> EHRVLHLRDRLDLAAELKLLCERGPLVRIPLEDGSAVHWFALGYDVVREVLGSEKFDKRVIGTHFNHQEMALPGNLLQLDPPEHTRLRRMVAPAYSVRRMQALEPRVQAIVDDHLDTMASTGPPVEFLREVAGPMAARVACEFLGIPLDDRGELIRLTAHRGGKRRRVLNGHAYLAYMRELAARLRRDPGDGMLGMVARDHGADISDEELAGLCAVVMNSSVEQTESCLAAGTLLLLEHPEQFALLRERPELGEQAVEEIVRYLSVFEGLDPRTATEDVEIGGQVIKKGEAVFCSLLAANRADPALDGFDITRKESRHVAFGHGIHHCLGAPLARMELRIAFTTLVSRFPSLRTAVPAEEIRFRPPSSNVFTLLELPLTW

Cytochrome P450 enzymes (P450s) are a superfamily of monooxygenases that utilize a cysteine thiolate–ligated heme moiety to perform a wide range of demanding oxidative transformations. Within GPA biosynthesis, P450s function in a specific, stepwise manner to install the essential side-chain crosslinks in the core peptide in a process that typically requires one Oxy enzyme per crosslink to be installed. Given the apparent preference for the unusual heme orientation shown by OxyA enzymes, we investigated the OxyA homolog from kistamicin biosynthesis (OxyAkis), which is an atypical GPA. Structural and biochemical analysis of OxyAkis has shown that this P450 enzyme is highly prone to oxidation and can display an atypical heme orientation in different protein batches.

With the general fold essentially unchanged, we performed a detailed analysis of the active site of this P450, which revealed a mixed population of heme orientations as seen in the Fo–Fc difference map electron density at the substituent vinyl and methyl groups. However, even once the density of the methyl/vinyl groups was well-explained by a mixture of heme orientations; there was still evidence for additional density at the side of the heme immediately below the I-helix (β-position). To explore the possibility of radiation damage to the heme due to long data collection causing this modification, we collected several datasets using an attenuated beam. Even with a beam attenuation of 95% and collecting data in small wedges to reduce possible damage, this dataset still showed density in the difference map for modification at the β-position of the heme.> SNAMKIALMMENSQAAKNAMVAGELNSVAGGLGHDVFNVGMTDENDHHLTYIHLGIMASILLNSKAVDFVVTGCGTGQGALMSCNLHPGVVCGYCLEPSDAFLFNQINNGNAISLAFAKGFGWAGELNVRYIFEKAFTGK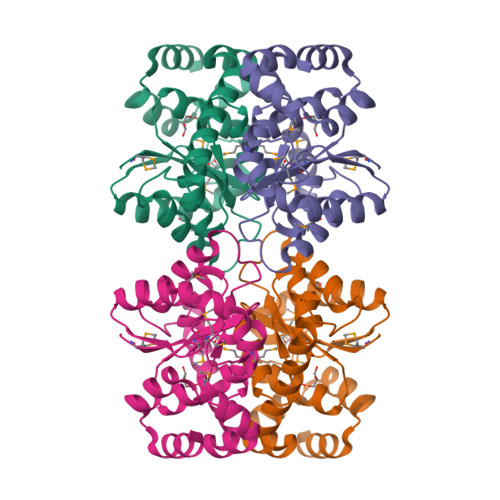RGEGYPIERAAPQQANAAILNNVKAAVAKDVVEGLRAIDQELVKTAVGSTQFQECFFAHCQVPEIAEYVKSLLD> TTKDVIQKGISVVGDLLGVVGFPFGGALVSFYTNFLNTIWPSEDPWKAFMEQVEALMDQKIADYAKNKALAELQGLQNNVEDYVSALSSWQKNPVSSRNPHSQGRIRELFSQAESHFRNSMPSFAISGYEVLFLTTYAQAANTHLFLLKDAQIYGEEWGYEKEDIAEFYKRQLKLTQEYTDHCVKWYNVGLDKLRGSSYESWVNFNRYRREMTLTVLDLIALFPLYDVRLYPKEVKTELTRDVLTDPIVGVNNLRGYGTTFSNIENYIRK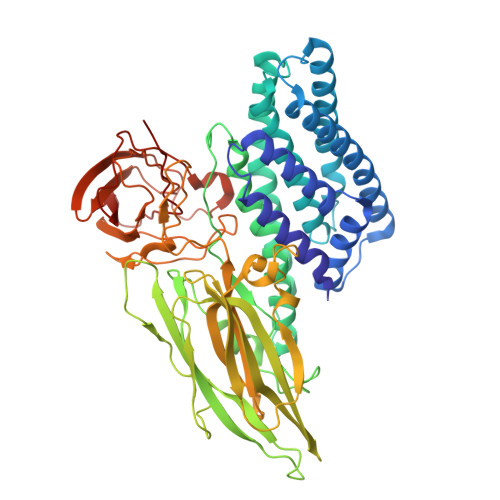PHLFDYLHRIQFHTRFQPGYYGNDSFNYWSGNYVSTRPSIGSNDIITSPFYGNKSSEPVQNLEFNGEKVYRAVANTNLAVWPSAVYSGVTKVEFSQYNDQTDEASTQTYDSKRNVGAVSWDSIDQLPPETTDEPLEKGYSHQLNYVMCFLMQGSRGTIPVLTWTHKSVDFFNMIDSKKITQLPLVKAYKLQSGASVVAGPRFTGGDIIQCTENGSAATIYVTPDVSYSQKYRARIHYASTSQITFTLSLDGAPFNQYYFDKTINKGDTLTYNSFNLASFSTPFELSGNNLQIGVTGLSAGDKVYIDKIEFIPVN> MPYDDVMTGSGFQRARSAQAKQQREEAILDAARELGTERGIREITLTDIAATVGMHKSALLRYFETREQIFLKITAEGWKEWSAELCARLRELPGAAPDAVGQVFAATLAARPLFCDLLAQAPLNLERNVSVESVRSFKIATLDEVGRIGAELRRLLGVDETQAVDVIATATSLAGALWQMATPGPHIQTLYRSDPRLAHAVVEVEPRLNRVLGALL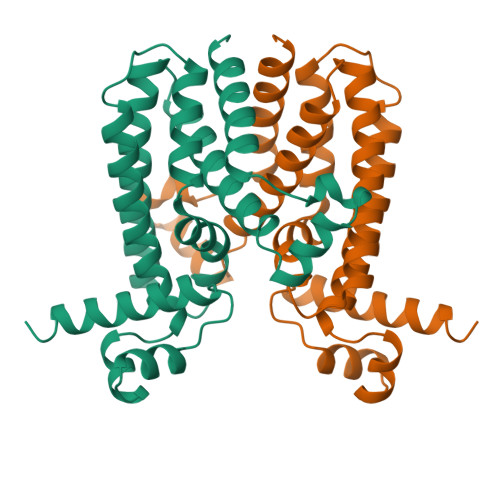RGIADGLEHHHHHH{3-chloro-4-[(3-{[7-propyl-3-(trifluoromethyl)-1,2-benzisoxazol-6-yl]oxy}propyl)sulfanyl]phenyl}acetic acid | C22 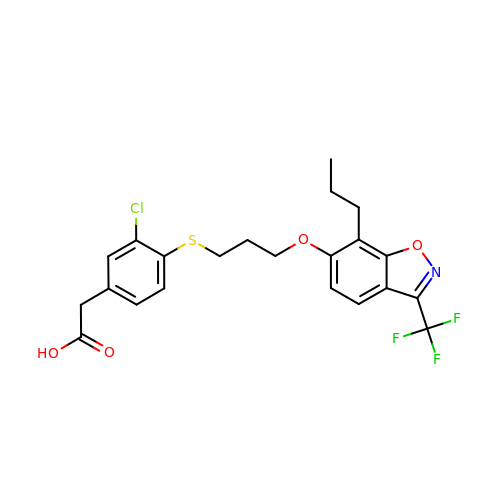H21 Cl F3 N O4 S | TZBRFAASYWFUGK-UHFFFAOYSA-N[(1~{S},2~{S},3~{S},4~{S})-2-(hydroxymethyl)-3,4-bis(oxidanyl)cyclopentyl] hydrogen sulfate | C6 H12 O7 S | 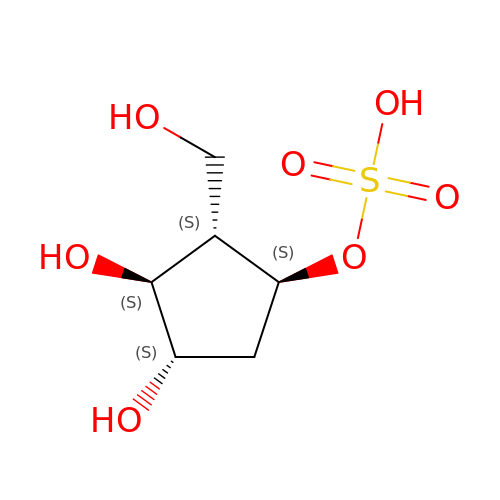WLWVVBPJYHXDMI-VANKVMQKSA-N> MASMTGGQQMGRGMAGPEIVKLKKILREKAVPPGTEVPLDVMRKGMEKVAFKAADDIQVEQVTVAGCAAEWVRAPGCQAGKAILYLHGGGYVMGSINTHRSMVGEISRASQAAALLLDYRLAPEHPFPAAVEDGVAAYRWLLDQGFKPQHLSISGDSAGGGLVLAVLVSARDQGLPMPASAIPISPWADMTCTNDSFKTRAEADPMVAPGGINKMAARYLNGADAKHPYASPNFANLKGLPPLLIHVGRDEVLLDDSIKLDAKAKADGVKSTLEIWDDMIHVWHA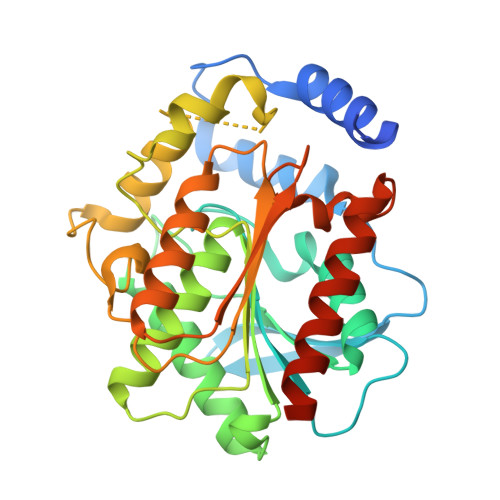FHPMLPEGKQAIVRVGEFMREQWAALAAALEHHHHHH>MKVAGVDEAGRGPVIGPLVIGVAVIDEKNIERLRDIGVKDSKQLTPGQREKLFSKLIDILDDYYVLLVTPKEIDERHHSMNELEAEKFVVALNSLRIKPQKIYVDSADVDPKRFASLIKAGLKYEATVIAEHKADAKYEIVSAASIIAKVTRDREIEKLKQKYGEFGSGYPSDPRTKEWLEEYYKQYGDFPPIVRRTWET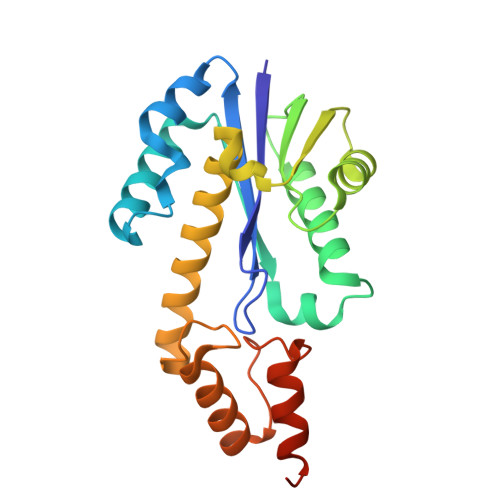ARKIEERFRKNQLTLDKFLK[2x]>MVLYFIGLGLYDERDITVKGLEIAKKCDYVFAEFYTSLMAGTTLGRIQKLIGKEIRVMSREDVELNFENIVLPLAKENDVAFLTPGDPLVATTHAELRIRAKRAGVESYVIHAPSIYSAVGITGLHIYKFGKSATVAYPEGNWFPTSYYDVIKENAERGLHTLLFLDIKAEK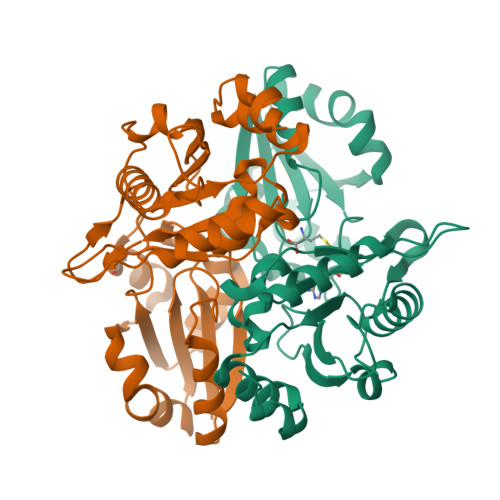RMYMTANEAMELLLKVEDMKKGGVFTDDTLVVVLARAGSLNPTIRAGYVKDLIREDFGDPPHILIVPGKLHIVEAEYLVEIAGAPREILRVNV[2x]>SNARGRLKVFLGAAPGVGKTYAMLQAAHAQLRQGVRVMAGVVETHGRAETEALLNGLPQQPLLRTEYRGMTLEEMDLDALLKAAPSLVLVDELAHTNAPGSRHTKRWQDIQELLAAGIDVYTTVNVQHLESLNDQVRGITG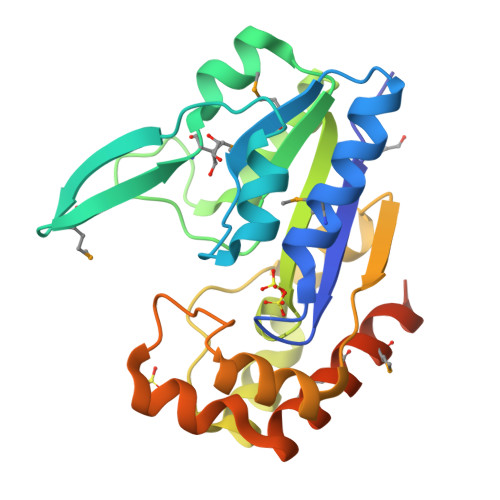VQVRETLPDWVLQEAFDLVLIDLPPRELLERLRDGKVYVPEQARAAIDAFFTQTNLTALREMAMQTAAAQVDNDLAQGYRQLGQSAP[2x]>MAPKRSRRSNRRAGSRAAATSLVYDTCYVTLTERATTSFQRQSFPTLKGMGDRAFQVVAFTIQGVSAAPLMYNAR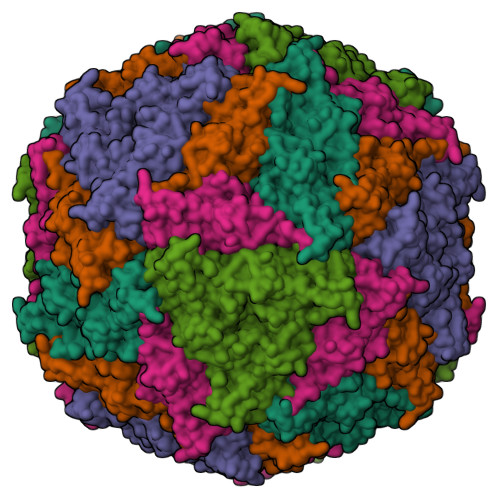LYNPGDTDSVHATGVQLMGTVPRTVRLTPRVGQNNWFFGNTEEAETILAIDGLVSTKGANAPSNTVIVTGCFRLAPSELQSS[5x]> GYSDRVRSLTLGNSTITTQESANVVVGYGRWPEYLRDDEATAEDQPTQPDVATCRFYTLESVQWEKNSAGWWWKFPEALKDMGLFGQNMLYHYLGRAGYTIHVQCNASKFHQGCLLVVCVPEAEMGCSQTDKEVAAMNLTKGEAAHKFEPTKTTGEHTVQSIVCNAGMGVGVGNLTIYPHQWINLRTNNCATIVMPYVNSVPMDNMFRHYNFTLMVIPFAPLDYAAQASEYVPVTVTIAPMCAEYNGLR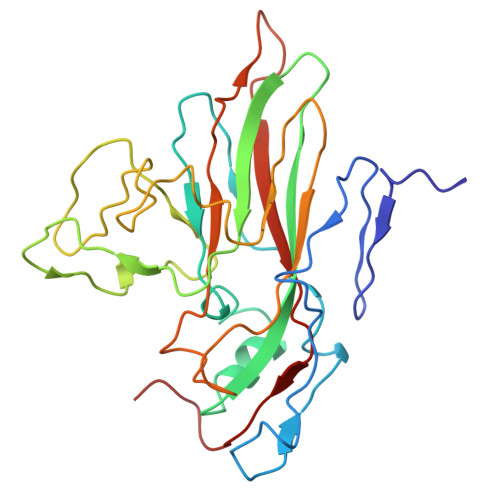LAYQQ>GHMADYKAPLRDMRFVLNEVFEVSRLWAQLPALAEVVDAETAAAILEEAGKVTAGTIAPLNRPGDEEGCQWNAGAVSTPAGFPEAYRTYAEGGWVGVGGDPAYGGMGMPKVISAQVEELVNSANLSFGLYPMLTAGACLALNAHASDELKDKYLPNMYAGIWAGSMCLTEPHAGTDLGIIRTRAEPQADGSYKISGTKIFITGGEHDLTENIIHLVLAKLPDAPAGPKGISLFLVPKVLVNADGSLGEKNSLGCGSIEHKMGIKASATCVMNFDGATGWLVGEVNKGLAAMFTMMNYERLGVGIQGLATGERSYQSAIEYARERIQSRAPTGPVAKDKAADPIIVHPDVRRMLLTMKALNEGGRAFSSYVAMQLDTAKYSEDAVTRKRAEELVALLTPVAKAFLTDMGLETTIHGQQIFGGHGFIREWGQEQLVRDCRITQIYEGTNGIQALDLVGRKVIGSGGAFSRHFTDEIKAFVASADEALGEFSKPLAAAVENLEELTAWLLDRAKGNPNEIGAASVEYLHVFGYTAYAYMWALMARTALAKQGEDDFYASKLGTARFYFARLLPRIHSLSASVRAGSESLYLLDAEQF[2x]

In this work, we identify the dominant fatty acyl-CoA dehydrogenases (designated FadE1 and FadE2, respectively) required for growth of P. aeruginosa on long- and medium-chain fatty acids. The resulting acyl-CoA enters the β-oxidation cycle, being initially converted to enoyl-CoA by an FAD-dependent fatty acyl-CoA dehydrogenase (FadE), followed by sequential hydration, oxidation, and thiolytic cleavage reactions. The FadE1 enzyme has a broad substrate specificity, being able to use both long- and medium-chain acyl-CoA substrates, whereas FadE2 exclusively uses medium-chain fatty acyl-CoAs. FadE1 (601 residues) and FadE2 (592 residues) had the same overall fold (with the backbone RMSD of 1.001 Å) as other acyl-CoA dehydrogenase (ACAD) superfamily members.

The structure of FadE1 and FadE2 were solved to a resolution of 2.08 Å and 1.94 Å, respectively. However, efforts to solve the FadE2 structure with a bound fatty acyl-CoA ligand failed. However, the substrate cavity of FadE2 was blocked in the middle, allowing FadE2 to only accommodate substrates with a maximum of 8-10 carbon atoms in the acyl chain. The blockage in the FadE2 substrate-binding cavity was due to the side chains of three amino acids; Met130, Glu296, and Gln303. In the crystal structure of FadE2, the side chains of Met130 and Glu296 protrude directly into the substrate channel, creating a physical block. Similarly, and although it is conserved between FadE2 and FadE1, the glutamine residue (Gln303) in FadE2 is oriented towards the substrate channel, whereas in the C16-CoA-bound FadE1E441A structure, the corresponding residue (Gln302) points away from the substrate-binding site. However, by comparing the substrate-bound FadE1E441A structure with that of apo-FadE2 (with no substrate bound) the analogous residues (Tyr440 and Tyr441, respectively) adopt an exclusively “open” configuration. Moreover, unlike the situation in FadE5Ms, where the loop containing Lys338 forms intimate contacts with the pantothenate moiety of the substrate, in both FadE1E441A and FadE2, this loop points away from the substrate. As previously noted, wild-type FadE2 was completely inactive against C16-CoA. One FAD molecule was bound in each protomer of FadE1 and FadE2.>KSMDIVVNDDLSCRFLEGFNTRDALCKKISMNTCDEGDPFFVADLGDIVRKHETWKKCLPRVTPFYAVKCNDDWRVLGTLAALGTGFDCASNTEIQRVRGIGVPPEKIIYANPCKQISHIRYARDSGVDVMTFDCVDELEKVAKTHPKAKMVL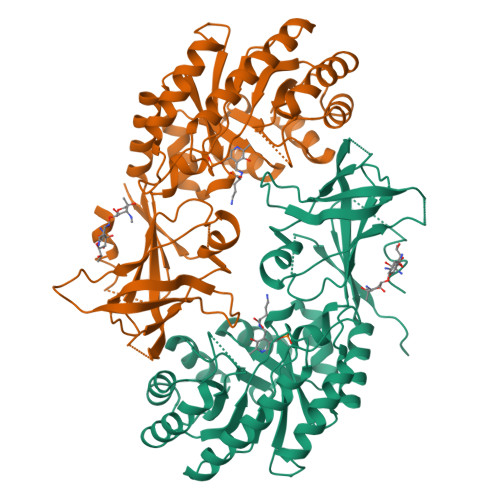RISTDDSLARCRLSVKFGAKVEDCRFILEQAKKLNIDVTGVSFHVGSGSTDASTFAQAISDSRFVFDMGTELGFNMHILDIGGGFPGTRDAPLKFEEIAGVINNALEKHFPPDLKLTIVAEPGRYYVASAFTLAVNVIAKKVTPGVQTDVGAHAESNAQSFMYYVNDGVYGSFNCILYDHAVVRPLPQREPIPNEKLYPSSVWGPTCDGLDQIVERYYLPEMQVGEWLLFEDMGAYTVVGTSSFNGFQSPTIYYVVSGLPDHVVRELKSQKS[4x]> ADKNPGSENMTNTIGPHDRGGSSPIYNILNSYLTAYNGSHHLYDRMSFLCLSSQNTLNGACPSSDAPGTATIDGETNITLQFTEKRSLIKRELQIKGYKQFLFKNANCPSKLALNSSHFQCNREQASGATLSLYIPAGELNKLPFGGVWNAVLKLNVKRRYDTTYGTYTINITVNLTDKGNIQIWLPQFKSNARVDLNLRPTGGGTYIGRNSVDMCFYDGYSTNSSSLEIRFQDDNSKSDGKFYLKKINDDSKELVYTLSLLLAGKNLTPTNGQALNINTASLETNWNRITAVTMPEISVPVLCWPGRLQLDAKVKNPEAGQYMGNIKITFTPSSQTLDNKQVEKNITVTASVDPVIDLLQADGNALPSAVKLAYSPASKTFESYRVMTQVHTNDATKKVIVKLADTPQLTDVLNSTVQMPISVSWGGQVLSTTAKEFEAAALGYSASGVNGVSSSQ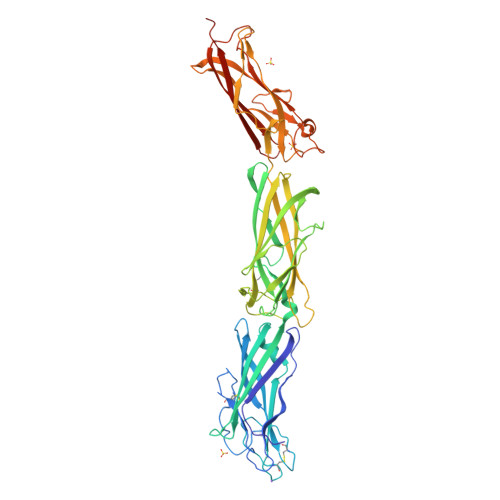ELVISAAPSTAGTAPTAGNYSGVVSLVMTLGSDNKQVEKNITVTASVDPVIDLLLEHHHHHH> YVDVGPDSVKSACIEVDIQQTFFDKTWPRPIDVSKADGIIYPQGRTYSNITITYQGLFPYQGDHGDMYVYSAGHATGTTPQKLFVANYSQDVKQFANGFVVRIGAAANSTGTVIISPSTSATIRKIYPAFMLGSSVGNFSDGKMGRFFNHTLVLLPDGCGTLLRAFYCILEPRSGNHCPAGNSYTSFATYHTPATDCSDGNYNRNASLNSFKEYFNLRNCTFMYTYNITEDEILEWFGITQTAQGVHLFSSRYVDLYGGNMFQFATLPVYDTIKYYSIIPHSIRSIQSDRKAWAAFYVYKLQPLTFLLDFSVDGYIRRAIDCGFNDLSQLHCSYESHHHHHH

The key determinant of host specificity is the envelope-located trimeric spike (S) glycoprotein, which can be further cleaved by host proteases into an N-terminal S1 subunit and a membrane-bound C-terminal S2 region. In the S1 subunit, the receptor binding domain (RBD, also called the C terminal domain, CTD) is localized in the C-terminal region, spanning ∼200 amino acids, and structural studies have revealed that the RBD consists of two subdomains: the core and external subdomains. For both MERS-CoV and SARS-CoV S proteins, the S2 subunit is mainly composed of α-helices and forms the stem region of the S protein. Here we present high-resolution structures of the trimeric MERS-CoV and SARS-CoV S proteins in its pre-fusion conformation by single particle cryo-electron microscopy (cryo-EM).

To date, little is known about the structural and functional information of NTDs for the MERS-CoV or SARS-CoV S proteins, though its counterparts from other CoVs, such as mouse hepatitis virus (MHV) and bovine coronavirus (BCoV), act as receptor binding domains and their crystal structures have already been delineated. We also solved the crystal structure of the RBD-preceding N terminal domain (NTD, residues 18–353) in the S1 subunit at a resolution of 1.5 Å. Our crystal and cryo-EM structures show that MERS-CoV and SARS-CoV NTDs fold into galectin-like structures as in BCoV, MHV and HKU1CoV. However, the glycan-binding site on the top of MERS-CoV NTD is occupied by a short helix and the N-linked glycan on that helix, and thus NTD in this conformation maybe unable to attach the cell surface by recognizing certain sugar molecules, unlike BCoV and HKU1. By contrast, the NTD domain is observed with strong and clear density, forming a stable triangular platform on the top of the S trimer. The flexible RBD regions are located on the triangular edges between the NTD domains. Since the RBD is located between the NTD domains, a strategy to develop neutralizing antibodies, which target the NTD and interfering with receptor binding through steric hindrance should be feasible in the future.> MATIVNTAAGAAVQRPRPRPGAERVLVCLSYCGGGTAPFRQWAEDLPEDVELALICYPGREARFGAPFARVWTELRDDVVRSVRGLTGRPYILFGHSMGSWMAFETAAELERIGAAPPEALVVSGGVAPHKRR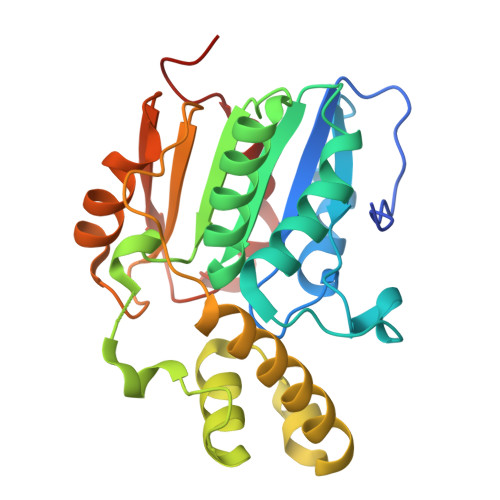EMPREDTPRSDADMDALVRWMRDLGQVSPAIAAEPELLKIAVDLLRADLAVTESYRFVDGTRVSVPLRVLYGTEDAAPFADVERHWRPLTAGPFQAVELPGGHFYTPEVWARLTEWCTLPVPGAAGTR CtfAB then transfers the CoA from acetoacetyl-CoA to acetate to reform an acetyl-CoA and produce acetoacetate. CtfAB is a member of family 1 CoA transferases. CtfB contains the acetyl-CoA binding site and the PS01724 signature sequence which includes the catalytic glutamate residue (E46) sandwiched between two short antiparallel beta strands on the N-terminal end of an eight-stranded mixed beta sheet. CtfA contains the acetate binding site and the PS01723 signature sequence.

Similar to other CoA transferases, acetyl-CoA is bound in an apparent high-affinity binding site in CtfB with most interactions occurring between the phospho-ADP of CoA and CtfB residues far from the acetate binding pocket. The binding site for acetyl-CoA involves primarily CtfB residues that are far from the catalytic glutamate where acetate is bound. For example, E46 CB is 25.5 Å from A146 CB. The adenosine base of acetyl-CoA is wedged between the methyl group of CtfB A146 (chain C) on one side and CtfB L158, I117, and L104 on the other side, shown in Figure 5. M121 extends the hydrophobic patch deeper into the binding site to make hydrophobic contacts with one methyl group of the pantothenic portion of CoA. The second pantothenic methyl group is positioned to make hydrophobic contact with L104. These extensive hydrophobic interactions are likely responsible for the high-binding affinity, but there are also several hydrogen bonds and electrostatic interactions as well. The acetyl-B-mercaptoethylamine group of acetyl-CoA is modeled only in the heterodimer cleft between chain C and chain D. In the chain A and B heterodimer, only the phosphoadenosine group is included in the model. There is 2Fo-Fc electron density for the modeled acetyl-B-mercaptoethylamine group between chains C and D, but the density includes multiple chain breaks and is weak in places. Interestingly, even with the acetyl-CoA group bound, there are two acetate molecules in the acetate-binding site. The shows difference density for two acetate molecules in the CtfAB F42TS45C-CoA structure. Acetate 1, colored magenta, is the only location where acetate is bound in the same conformation in each structure.

>[2x]MKVVDISKINELVKEGATLMIGGFLGVGTPENIIDEIIRHNISNLTVIANDTAFEDRGIGKLVKNKLCKKVIVSHIGTNPETQRQMIEGTLEVELVPQGTLAERIRAAGVGLGGILTPTGVGTVVEKDKKVIEVEGKKYLLELPIHADVALIKAKKADYLGNLVYNLTAENFNPIMALAAKTVIAEVEEIVPTGTLSPNEIKTPGIIVDYIVTGVTR;>[2x]MNPKEKIAIRVAQELKKGQLVNLGIGLPTLVANYIPKDIHVTFQCENGIIGMGPAPKEGYENSDLTNAGASYITALPGAMTFDSAFSFGIIRGGHLDVTVLGGLQVDEEGHLANWMIPGKMIPGMGGAMDLVTGAKKVIVAMTHTAKGTPKIVKKCTLPLTSIRKVDLIVTELAVIEPTDEGLLLKEISKETTLDEVLKLTEAKLIIADDLKIFA>SDKLELLLDIPLKVTVELGRTRMTLKRVLEMIHGSIIELDKLTGEPVDILVNGKLIARGEVVVIDENFGVRITEIVSPKERLELLNE[2x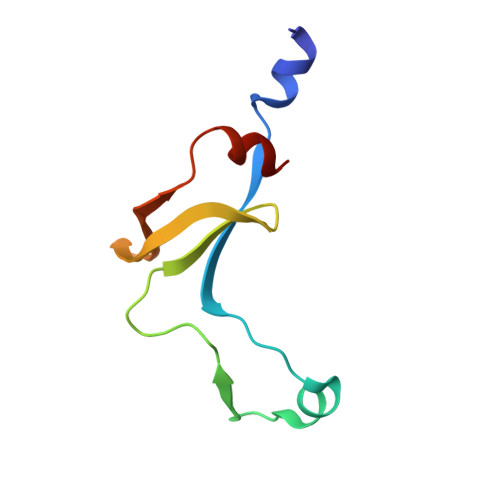]>GIDPFTMTPSEDFVVTDRGGIVENSHRVHAAVVDAKGRLLYALGNPTRMTLARSAAKPAQALAILETEGVAGYGFDDADIALMCASHSSEDRHIARTRAMLSKIKAEEADLRCGGHPSLSEMVNRSWIKQDFIPTAVCSNASGKHVGMLAGARAIGAGTDGYHLPDHPMQGRVKRTVAELCDLDAGDVEWGTDGCNLPTPAFPLDRLGRIYAKLASAADGSDAGEGQSTRCAALAHIFRAMARHPEMVAGEGRYCTMLMRAFDGALVGKLGADASYAIGVRASDATRQLGTDGALGISVKIEDGNLEMLYAVVTELLERLGIGSPDVRSQLASFHHPQRVNTMGVTTGGVSFPFKLRGSKSNVDDPRLAAVAR[2x]

Asparaginases (EC 3.5.1.1), which split L-asparagine to L-aspartate and ammonia, are grouped into three unrelated structural classes: Class 1 (bacterial-type), Class 2 (plant-type), and Class 3 (Rhizobium etli-type). ReAV is a homodimer with an α/β protomeric fold, formed by two tightly packed domains. The active site of the enzyme is located in a cleft on the protomer surface and marked by a zinc ion with an unusual coordination sphere created by Cys135, Lys138, Cys189, and a water molecule. The conspicuous catalytic center of the enzyme comprises two Ser-Lys tandems (Ser48-Lys51 and Ser80-Lys263), centered around the curiously hydrated Ser48 residue and located in the close vicinity of the metal binding site.

The crystal structure of this mutant revealed that the absence of Cys135 caused small structural rearrangements in the active site area, almost identical in the two subunits of the dimer, and triggered a collapse of the metal coordination site, since the mutant protein was unable to bind the Zn2+ cation. This disability was additionally confirmed by ITC affinity studies. The hydration pattern of Ser48 is nearly identical as in the WT protein, with three tightly bound water molecules in the close vicinity of the Ser48 hydroxyl group. These water molecules form strong hydrogen bonds with the Ser48 Oγ atom, with O…O distances in the range of 2.4–2.7 Å. In the close vicinity of these waters and Asp187, we observed a bound polyethylene glycol chain in subunit A or a glycerol molecule in subunit B, both located at the exit of the putative active site. The side chain of Ser48 is H-bonded to the Nζ atom of Lys51 and the Oγ atom of Ser80. The pattern of H-bonds at the two lysine residues from the Ser-Lys tandems, Lys51 and Lys263, is roughly the same as in the WT protein. Only one conformer of Asp187 is visible in the electron density maps, with one of its Oδ atoms forming an H-bond to the Nε atom of Arg47. Interestingly, the side chain of Cys249 does not carry its typical chemical modification, which may be linked to the absence of the Zn2+ cation in the protein structure. The structures of the C135A and C189A mutants demonstrate that alanine substitution of the cysteine residues involved in zinc coordination led to collapse of the metal binding site and abrogation of the L-asparaginase activity.>[2x]MPVLENRAAQGDITAPGGARRLTGDQTAALRDSLSDKPAKNIILLIGDGMGDSEITAARNYAEGAGGFFKGIDALPLTGQYTHYALNKKTGKPDYVTDSAASATAWST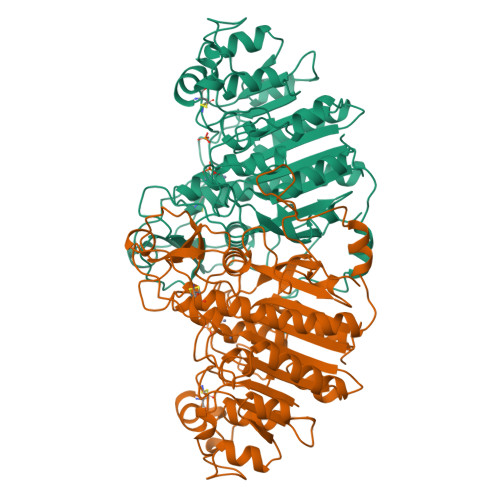GVKTYNGALGVDIHEKDHPTILEMAKAAGLATGNVSTAELQHATPAALVAHVTSRKCYGPSATSEKCPGNALEKGGKGSITEQLLNARADVTLGGGAKTFAETATAGEWQGKTLREQAQARGYQLVSDAASLNSVTEANQQKPLLGLFADGNMPVRWLGPKATYHGNIDKPAVTCTPNPQRNDSVPTLAQMTDKAIELLSKNEKGFFLQVEGASIDKQDHAANPCGQIGETVDLDEAVQRALEFAKKEGNTLVIVTADHAHASQIVAPDTKAPGLTQALNTKDGAVMVMSYGNSEEDSQEHTGSQLRIAAYGPHAANVVGLTDQTDLFYTMKAALGLK> MNVKETKLEDVLKSRGIDMKDAYNISEADIPEAKESTQKLMDIYYTLKVTADMEAAYWYNRTWWENDGEVIEVRRAKAVAASLSHMTPTILPYEKLVMNKTKNVRGAFPFPWVCASFFNAQAEALMNEVDAPAENEADSVSVVGAGGGNVTESYGNVISIAKKFGMRKEEIPVLVKTSKPWEGISVEELSNKYSKMTPGYDQFKNIMESVICMFDSFAIPQGREVINYYMPLQYGFDGIIKLCDEKIAEVMGEAGDDGDFGMSRGYYYAAMKEITKGLSAWCENYSKRAKYLASIETDSEIKANYEKIEEVMGNIAHKKPANFWEAIQMTLCCHFGVVNEDPQSGLSIGRLGQVLQPFYEKDVEDGIMTDEEVIELLELYRIKITCIECFASAGVSGGVLSGNTFNNLSLGGQNYDGLSAVTPLEYLIVEAGMRNQTPQPTLSVLYDEKTPEDFLMKAASCTKLGLGYPAWMNNQTGMNFMMRNYGPEGMDLHDARAWCLGGCLESAPGCFLPLEYNGKVTMIPGGASPTCGTGVHFIGMPKVLELVLTNGLDKRTGKQVYPPHNKKLDSYETMVNQWKEYMELTTDVVNRCNNIQMDIWRKYNMPAVNSLLKPDCFKKGKHIGTMGARYNSCINFESCGTITFVNSLSSIKKNVFDDSKFTIEEM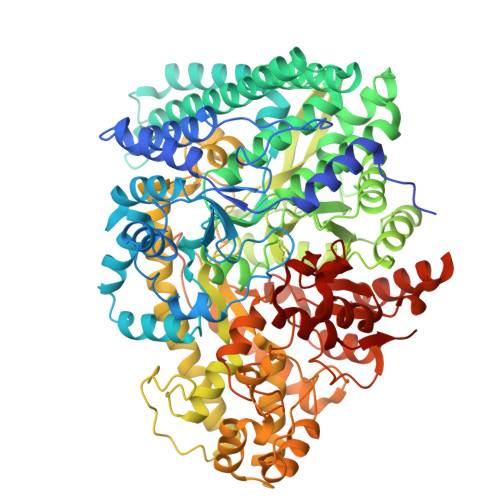TDAMLNNFGFKTAYETEVFSPDFRESTDKSTKYEKIFAACVNAPKYGNADKYADEIFKAYHYYIYDMTHKFRSYYGKPLYLCQISVSTHGPQGFVTLATADGRLAGTTYSDGSVSAAAGTDKNGIYAIFESATVYDHSMHQNAQMNLKLHPTAVKGINGTRKLLDLVRAYMRKGGFHVQFNVVDSKTLRDAQLTPEKYRELMVRVAGFTQYWCEIGKPIQDEVIYRTEYDK>MGHHHHHHSHMQNADDFIKFLELEQHVEGGFYRSSYRSE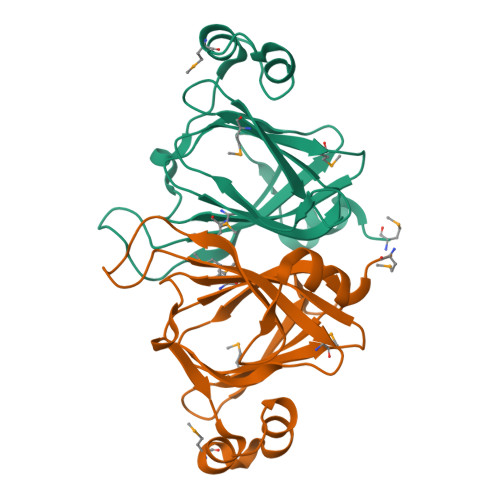TAFDPSRQLWSSIYFLLRTGEVSHFHRLTADEMWYFHAGQSLTIYMISPEGELTTAQLGLDLAAGERPQFLVPKGCIFGSAMNQDGFSLVGCMVSPGFTFDDFELFSQEALLAMYPQHKAVVQKLSRPEVN[10x]2-amino-7-phenyl-3-{[(2R,5S)-5-phenyltetrahydrofuran-2-yl]methyl}quinazolin-4(3H)-one 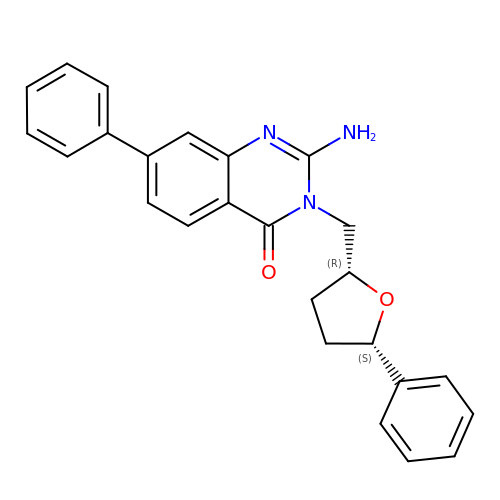| C25 H23 N3 O2 | ZFQQCJCOZGMLDR-OFNKIYASSA-N>[2x]C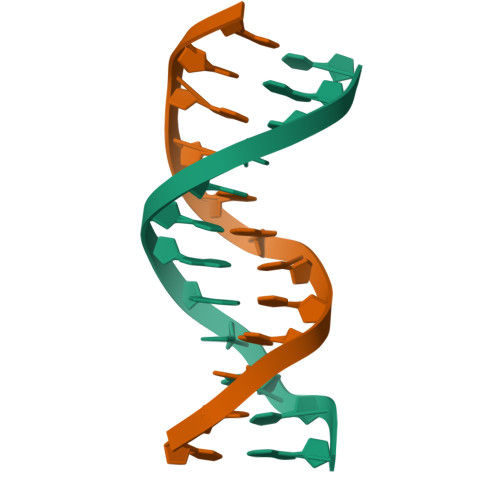GCGTTAACGCG> MGGSHHHHHHENLYFQG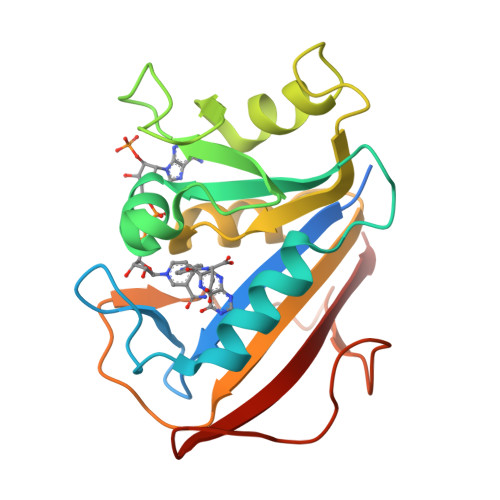MVGSLNCIVAVSQNMGIGKNGDLPWPPLRNEFRYFQRMTTTSSVEGKQNLVIMGKKTWFSIPEKNRPLKGRINLVLSRELKEPPQGAHFLSRSLDDALKLTEQPELANKVDMVWIVGGSSVYKEAMNHPGHLKLFVTRIMQDFESDTFFPEIDLEKYKLLPEYPGVLSDVQEEKGIKYKFEVYEKND> GTTGGGGTTGGGGTTGGGGTTGGGGT

G-quadruplexes (GQs) are non-canonical DNA structures composed of stacks of stabilized G-tetrads. Telomeres are repetitive, G-rich DNA sequences that exist at the ends of linear chromosomes and aid in their stabilization and protection. In this work, we focus on the telomeric repeat from Tetrahymena thermophila (referred to as TET) which has the overall sequence (TTGGGG)n. Furthermore, we report four high-resolution K+-stabilized crystal structures of two variants, TET25 (one structure) and TET26 (three structures).

PAGE gel on TET26 crystals and crystal structures of all three forms of TET26 revealed that only the parallel four-tetrad GQ crystallized. TET26 has three propeller TT loops as well as 5′-GTT and 3′-T overhangs. All guanines adopt anti glycosidic conformations, as is expected for parallel GQs. In each case, the ASU contains one GQ monomer which forms a 5′-5′ crystallization dimer with a symmetry generated partner. The monomers can be classified as type VIII-1a GQs with four medium grooves of an average dimension of 14.6 ± 0.1 Å, Supplementary Table S7 and Supplementary Figure S7B. The 3′-end K+ ion is located closer to the terminal tetrad with an average K–O distance of 2.63 ± 0.03 Å compared to 2.92 ± 0.02 Å from the middle tetrad. This is likely due to the relatively high non-planar deformation of the 3′-tetrad (DOOP= 1.83 Å) which leads to a larger opening in its center. All K+–K+ distances are in the range of 3.22–3.31 Å. The ion channel is extended in the 3′ direction by a water molecule located 3.19 Å away from the 3′-end K+, Supplementary Figure S10.> SRANDAPIVLLHGFTGWGREEMFGFKYWGGVRGDIEQWLNDNGYRTYTLAVGPLSSNWDRACEAYAQLVGGTVDYGAAHAAKHGHARFGRTYPGLLPELKRGGRIHIIAHSQGGQTARMLVSLLENGSQEEREYAKAHNVSLSPLFEGGHHFVLSVTTIATPHDGTTLVNMVDFTDRFFDFQKAVLKAAAVASNVPYTSQVYDFKLDQWGLRRQPGESFDQYFERLKRSPVWTSTDTARYDLSVPGAEKLNQWVKASPNTYYLSFATERTYRGALTGNYYPELGMNAFSAVVCAPFLGSYRNATLGIDDRWLENDGIVNAFSMNGPKRGSTDRIVPYDGTIKKGVWNDMGTYNVDHFEVIGVDPNPLFDIRA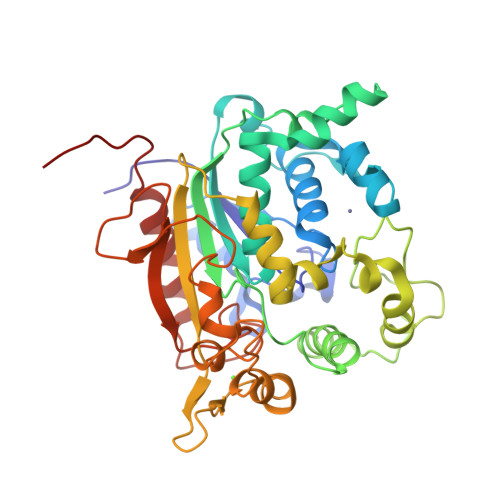FYLRLAEQLASLQPHHHHHH>[2x]MAGQSTHYLAFPRASTITWGDDTRYWSWATVDFCSYAIEEARLLQVSWLDCRWSMDASDFKQDI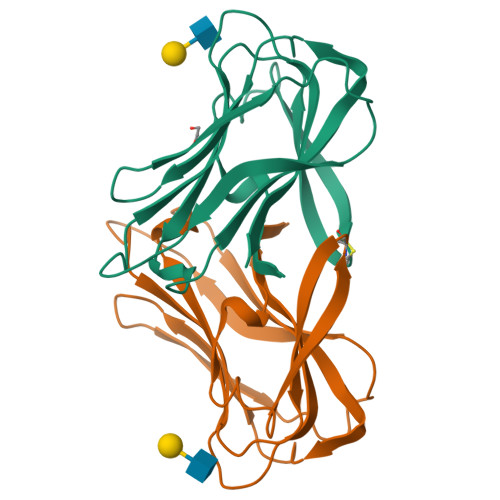WYNASVEVMLTSNASGWNVPLHLEIELPDGSKQESQIVLAGRQPNVWFKIPIGKFILRGSLTSGTIRFGFYNHEGNWKRGLNIRILAIQA> GPGMKQKIVIKVPMASDKCRS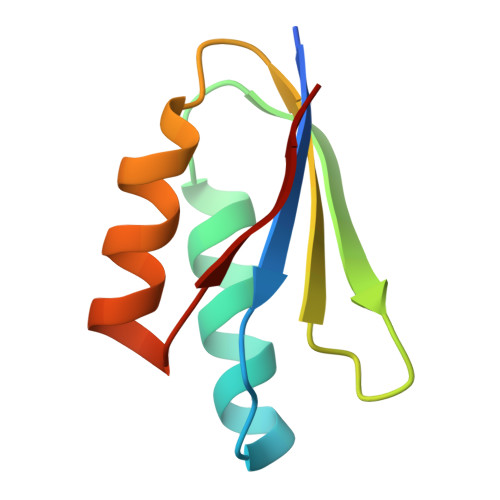KAMALVASTGGVDSVALVGDLRDKIEVVGDGIDSIKLVSALRKKVGHAELLQVS> GNSDDARTSIEQRSNAVSQVLLGIFSYVRWPKEPAVLQLCVVGPTEYADGLLRGMVQANGRRVHAERRAVDNPD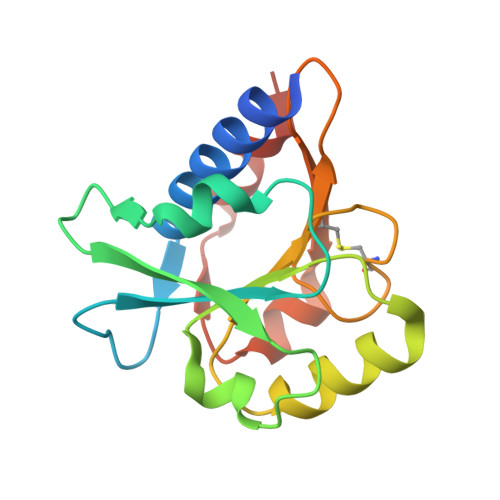LGTLCNVIYLGVVDERERQQVFRSLAGHPVLSISERGTECSVGSMFCLNVGGPRITFEANLDSIARSGVRVHPSVLKLARRQATP>[2x]XGEIAQAIKEIAKAIKEIAWAIKEIAQAIKGX

CCs are quaternary structures comprising two or more α-helices supercoiled around each other with cyclic (Cn) or dihedral (Dn) symmetry. Here, we describe variants with all combinations of the aliphatic residues, Ile, Leu and Val, at a and d to give four classes of peptide: the ββ class, with a and d = Ile or Val; Lβ, a = Leu and d = Ile or Val; βL, a = Ile or Val and d = Leu; and LL, a = d = Leu. Peptides are named systematically appending the one-letter code for the amino acids at the a and d sites to “CC-Type2-“; e.g., CC-Hept becomes CC-Type2-LI. In summary, solution-phase data and X-ray crystal structures demonstrate conclusively that different classes of Type-2 coiled-coil (CC) peptides—i.e., based on abcdefg repeats with predominantly hydrophobic residues at a, d, e and g—adopt a range of distinct states.

As a = d = β-branched specify blunt-ended α-helical barrels, we explored all four combinations of Ile and Val at these sites. CC-Type2-VV, -IV, -VI and -II, were helical and bound DPH in solution consistent with α-helical barrels. Interestingly, X-ray crystallography revealed that oligomer state increased through this series: CC-Type2-VV was hexameric; CC-Type2-IV, heptameric; and CC-Type2-II, octameric. The latter extends the range of discrete water-soluble α-helical barrels presented to date; though we note that the solution-phase and solid-state oligomers states do not match for this particular peptide. Concomitantly, the dimensions of the internal pore diameters increased: VV, 4.8–7.7 Å; IV, 6.2–9.2 Å; and II, 9.0–11.0 Å. Inspection of the models for these alternative states exposed steric clashes associated with the β-branched residues; e.g., threading of the CC-Type2-II sequence onto the CC-Type2-LL-Sg structure resulted in irreconcilable clashes between Cδ and Cγ1 atoms of Ile residues at a and d’ sites of neighbouring helices. More specifically, by disfavouring alternative states, potential steric clashes involving β-branched Ile residues at a and d appear critical for maintaining parallel α-helical-barrels structures.> ADAPGDDYVISAPEGMKAKPKGDKPGALQKTVPFPHTKHATVECV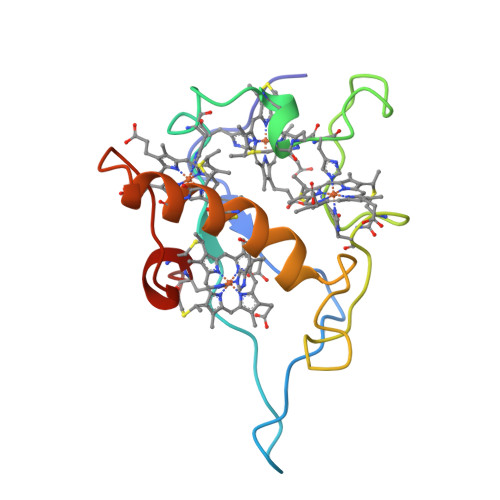QCHHTLEADGGAVKKCTTSGCHDSLEFRDKANAKDIKLVENAFHTQCIDCHKALKKDKKPTGPTACGKCHTTN> MGMVVALGLAFGTSGARAIACDFDSDRSVSVSVTFPKTSQNWPQVWREALWQLLTQIPADWRSRIERIAIDGTSGTVLLCDREGQPQTEPLLYNQACPIDLADLADWVPADHAALSSTSSLAKLWFWQQQFGALPPDWQILAQADWLSLQLHGCSQQSDYHNALKLGYSPDRERFSKNLLDSELGALLPVVHEPGVAIGPILPAIAQEFGLSPDCQICAGTTDSIAAFLASGAHQPGEAVTSLGSTIVLKLLSQVAVSDRLTGVYSHKLGGYWLTGGASNCGGATLRQFFPDTELESLSCQIDPTKKSGLDYYPLPSRGERFPIADPDRLPQLEPRPENPVQFLQGLLEGLTQVETLGYQRLQDLGATPLKRIWTAGGGAKNAVWQQLRQQAIGVPIAIAPNTEAAFGTARLAAFGLAAFHSAGLKRTLEHHHHHH

Synpcc7942_2462 from the cyanobacteria Synechococcus elongatus PCC 7942 encodes a putative sugar kinase (SePSK), and this kinase contains 426 amino acids. The At2g21370 gene product from Arabidopsis thaliana, xylulose kinase-1 (AtXK-1), whose mature form contains 436 amino acids, is located in the chloroplast (ChloroP 1.1 Server). SePSK and AtXK-1 display a sequence identity of 44.9%, and belong to the ribulokinase-like carbohydrate kinases, a sub-family of FGGY family carbohydrate kinases. Domain I exhibits a ribonuclease H-like folding pattern, and is responsible for the substrate binding, while domain II possesses an actin-like ATPase domain that binds cofactor ATP.

Our results suggested that three conserved residues (D8, T11 and D221 of SePSK) play an important role in SePSK function. To identify the function of these three residues of SePSK, we constructed D8A, T11A and D221A mutants. Using enzymatic activity assays, we found that all of these mutants exhibit much lower activity of ATP hydrolysis after adding D-ribulose than that of wild type, indicating the possibility that these three residues are involved in the catalytic process of phosphorylation D-ribulose and are vital for the function of SePSK. Our SePSK structure shows that the Asp8 residue forms strong hydrogen bond with RBL2. In addition, our enzymatic assays indicated that Asp8 is important for the activity of SePSK. To further verified this result, we measured the binding affinity for D-ribulose of both wild type (WT) and D8A mutant of SePSK using a surface plasmon resonance method. The results showed that the affinity of D8A-SePSK with D-ribulose is weaker than that of WT with a reduction of approx. two third. Dissociation rate constant (Kd) of wild type and D8A-SePSK are 3 ms-1 and 9 ms-1, respectively. The results implied that the second RBL binding site plays a role in the D-ribulose kinase function of SePSK.> LNPEQVAKIGAAIDAGRKYLDAKIEEAKKTLTLRTAQALLVIRSQYERAVDTLFTDPSAAEKELAATLATIDRLL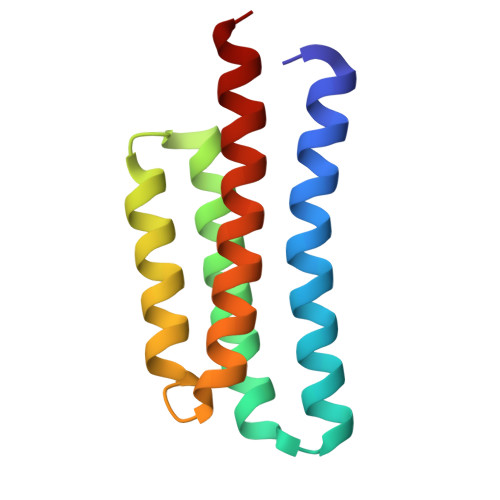KEHPELAAEIKAFIRSTMAEIRALLAASLAA>[2x]MAHHHHHHMKSIAQEHDCLLIDLD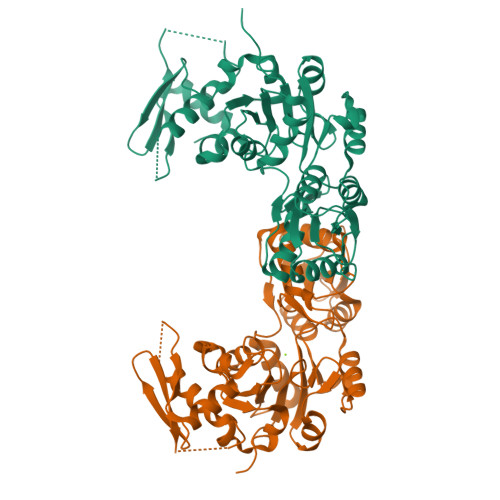GTVFCGRQPTGGAVQSLSQVRSRKLFVTNNASRSADEVAAHLCELGFTATGEDVVTSAQSAAHLLAGQLAPGARVLIVGTEALANEVAAVGLRPVRRFEDRPDAVVQGLSMTTGWSDLAEAALAIRAGALWVAANVDPTLPTERGLLPGNGSMVAALRTATGMDPRVAGKPAPALMTEAVARGDFRAALVVGDRLDTDIEGANAAGLPSLMVLTGVNSAWDAVYAEPVRRPTYIGHDLRSLHQDSKLLAVAPQPGWQIDVGGGAVTVCANGDVDDLEFIDDGLSIVRAVASAVWEARAADLHQRPLRIEAGDERARAALQRWSLMRSDHPVTSVGTQ> MTKPEILQLGPYPAWDQEPLDAAFTVHRLFEADDRAAMLANVGDRIRAIATRGELGASRALIEACPNLELISVYGVGYDAVDLAACRERGIQVTNTPDVLTGDVADLGVAMMLAQSRGIIGAETWARSGKWAAEGLYPLKRRVFGR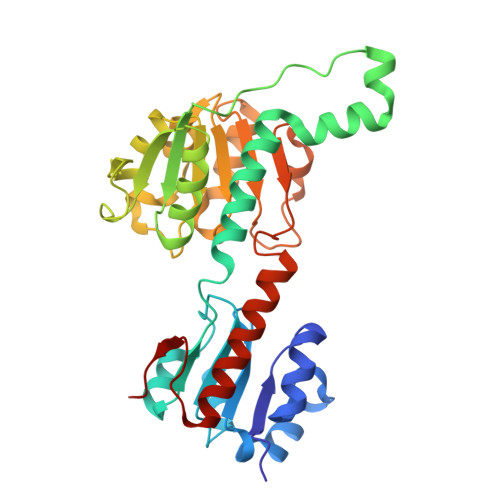RAGVLGLGRIGFEVARRLAGFDMQISYSDIAPKSYAPDWTFVEDAVTLARDVDFLFVTLAASAATRHIVGRDVIEALGPEGMLINISRASNIDEEALIAALADGRLGSAALDVFEGEPNFDPRFRDLPNVLLQPHHASGTIETRKAMGQLLRDNLTAHFAGSPLLTPVVLEH>RADPDPMKNTCKLLVVADHRFYRYMGRGEESTTTNYLIELIDRVDDIYRNTAWDNAGFKGYGIQIEQIRILKSPQEVKPGEKHYNMAKSYPNEEKDAWDVKMLLEQFSFDIAEEASKVCLAHLFTYQDFDMGTLGLAYGGSPRANSHGGVCPKAYYSPVGKKNIYLNSGLT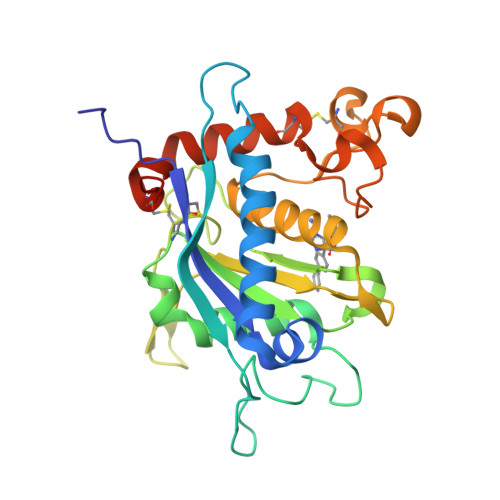STKNYGKTILTKEADLVTTHELGHNFGAEHDPDGLAECAPNEDQGGKYVMYPIAVSGDHENNKMFSQCSKQSIYKTIESKAQECFQERSNKGSHHHHHH[2x]> MKIAVIGQSLFGQEVYKELKNEGHMIVGVFTIPDKDGKVDPLAIEAEKDGVPVFKFPRWRLKGKAITEVVDQYKAVGAELNVLPFCSQFIPMEVIDHPKHGSIIYHPSLLPRHRGASAINWTLIHGDKKGGFTVFWADDGLDTGPILLQRECDVEPNDNVNSIYKRFLFPEGVKGMVEAVRLIATGKAPRIKQPEEGATAECIQKKENSKIDWNQPAEAIHNWIRGNDRVPGAWAEIDGKSVSFYGSTLLENDHFSSNGQPLEIPGASRAALVTKNGLVLFGNDGKMLLVKNLQFEDGKMIPGSQYFKAGVEHHHHHH

10-Formyltetrahydrofolate dehydrogenase (FDH), which is composed of a small N-terminal domain (Nt-FDH) and a large C-terminal domain, is an abundant folate enzyme in the liver and converts 10-formyltetrahydrofolate (10-FTHF) to tetrahydrofolate (THF) and CO2. Nt-FDH alone possesses a hydrolase activity, which converts 10-FTHF to THF and formate in the presence of β-mercaptoethanol. The N-terminal hydrolase domain of FDH (Nt-FDH) binds folate and is homologous to glycinamide ribonucleotide formyltransferase (GART) and methionyl-tRNA formyltransferase (FMT), enzymes that are crucial for de novo purine biosynthesis and translation initiation, respectively. In this study, we determined crystal structures of zebrafish wild-type apo Nt-FDH (zNt-FDH) and its ternary complexes with the substrate 10-formyl-5,8-dideazafolate (10-FDDF) and the products tetrahydrofolate (THF) and formate.

The catalytic mechanism underlying the hydrolase reaction is also suggested based on comparative analysis of the zNt-FDH Y200A mutant and the structural alterations associated with substrate and product binding. Phe89, Arg114 and Tyr200 are highly conserved in FDH from all species. The activity assay shows that the hydrolase activities of the F89A, R114A and Y200A zNt-FDH mutants decreased significantly in comparison to that of zNt-FDH_WT. As expected, the Y200A mutation decreased the enzymatic activity by ∼62%, preventing us from examining the kinetic properties of the mutant FDH. We co-crystallized or soaked crystals of the mutant (Y200A) with the product THF, but we observed no clear extra electron density in the active sites of the structures. Our results suggest that Tyr200 might play a crucial role in the release of products. Finally, from our structures, we have identified a new key residue Tyr200 that might be involved in product release, product inhibition and additional THF binding.We reveal the cryo-electron microscopy structure of a type IV-B CRISPR ribonucleoprotein (RNP) complex (Csf) at 3.9-Å resolution. The complex best resembles the type III-A CRISPR Csm effector complex, consisting of a Cas7-like (Csf2) filament intertwined with a small subunit (Cas11) filament, but the complex lacks subunits for RNA processing and target DNA cleavage. Surprisingly, instead of assembling around a CRISPR-derived RNA (crRNA), the complex assembles upon heterogeneous RNA of a regular length arranged in a pseudo-A-form configuration. These findings provide a high-resolution glimpse into the assembly and function of enigmatic type IV CRISPR systems, expanding our understanding of class I CRISPR-Cas system architecture, and suggesting a function for type IV-B RNPs that may be distinct from other class 1 CRISPR-associated systems.

The type IV-B complex resembles a sea cucumber, with six Csf2 (Cas7-like) subunits forming a helical “backbone,” and five Cas11 subunits comprising a helical “belly”. Each Cas11 subunit sits upon a Csf2-Csf2 interface. The “α-helix bundle” topology of Cas11 and presence of a contiguous positively-charged patch running along the length of the minor filament are typical of Cas11 small subunits in class 1 CRISPR systems (Rollins et al., 2019; Xiao et al., 2017), although the arrangement of helices within type IV Cas11 is distinct from type I and type III small subunits. Like other class 1 Cas7 proteins, Csf2 adopts a hand-shaped structure with fingers, a palm, and a thumb. The palm makes extensive contacts with the bound RNA (buried surface area of ∼1200 Å2 per Csf2 subunit), while the thumbs of neighboring Csf2 subunits protrude into the center of the palm, inducing a kink in the RNA backbone and a “flipped” base at six nucleotide intervals (typical of other class 1 complexes (Jackson et al., 2014; Taylor et al., 2015)). Csf2 subunits are intimately connected (1021 Å2) and make a network of contacts with bound RNA (∼1200 Å2 buried surface area per Csf2 subunit). (F) Cas11 binds at the interface with buried surface area of 505 Å2 (150 Å2 and 355 Å2 with Csf2.3 and Csf2.4, respectively). Csf2 had significant similarity to the type III-A CRISPR Csm3 (i.e. Cas7) subunit (Dali Z score of 14.1), despite a sequence identity of only 16%. Csf2 and Csm3 superimpose with an r.m.s.d of 2.9 Å and use equivalent interfaces to bind RNA and induce near-identical RNA backbone conformations (r.m.s.d of 1.5 Å). Although the M. sp. JS623 type IV-B operon contains both Csf3 (Cas5) and the putative large subunit Csf1, we did not observe corresponding densities within the high-resolution cryo-EM structure.

>[6x]MSWSHPQFEKGAMTLSTIRWDVDIIAQSSIVHRDDYTSVGSDTFTLFRREKIIGPDGQILQIPLISGSSFRGVLRRVGEALTAEVLGYEDVALPVPAAHLLTNGGRLAKSAHPLTDEEERNLKELLPQIAVFGGAASGRVMSGLLSVSKVLPEIAELAHLLPRPPHSTPLLPAVLSVADESFTHLPDHRPSTGGAPRTDHADGSPLGRFAIETLPAGTRLQTWARLDNATEHQAAFFDNVLSTFAAHGHLGGRSAAGHGQVTATVTATALRGSLPRPTVDWVNQLADDRDAAIAALTRLT;>[5x]MTTPTPTQVWRATVPELPPLVDEAGDTGSATARAADTAERLLLLLHYSIDWESSWVADPKHRKTYWDELLPGRVRRAAYRADTLDRWWSEVAGQLGAPAPRHRDRRLELATLLREPALPVITVLRDSLPALLLRVRIIAEAVAAQRGNNSAATSSADPNEPA>MYFFSVDPRNGASSVDACGKCCCESISARPGEVNGVMVSYVAWSAPLGGHGLTNKTTFEFENVSVTEPLVNSAFERTPFNTTLAGSLAALFPNPEGEAVEYEILELYPPVNGIVELGENGAFTYRPATSFTGIDRFWFSINGNVGEFVIAVDPAQGPQIAQPPFTPAVYVPLSRREVNKQTQALRFVLGVSPAAKPADIYRLNIRQAAIDCEGNEYFH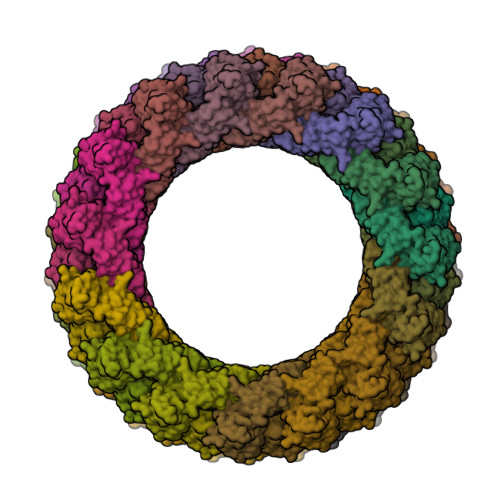ISCYDISIGSCG[60x]tricarbonodiimidic diamide 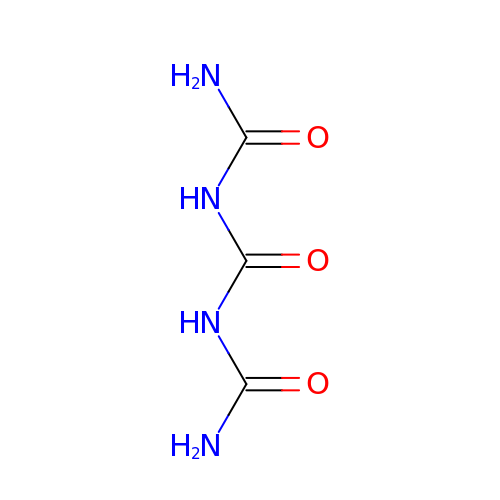| C3 H6 N4 O3 | WNVQBUHCOYRLPA-UHFFFAOYSA-N>MEASVSFENGKIVVRLPITRPTSKIAVKKIENGVGIPVSTRKKSFPSDENLRDYYIAWQISYARDGKYDYELSRMVRLAHEHGILTYNDIYELLKFADDVKSYLEDKGIRRESTNEELYGFNIYEDVYPVAKKELPSGEFIGIVLKHKQRAVGYQSMVYVCIPLTNVEPS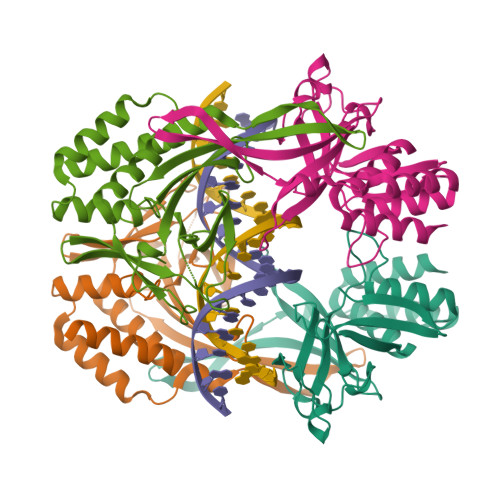LAGRVARRNEVVKYEVPVDLMKELLKAFIIASETHKNDIVKFLRSIIGTS[2x]> MGFSAEQAKKDGKDQSPVSESSSVGGTSPATASSVVSPNEPKLSGKEAKALKKARKQASRRAKAEAAAANNPPGVSEEKKVAIPNKNSNQQKKASKQNPQNSPETDANLQEKKIFEEKQVSIFSHLDWRRRRTTENIPKDIHPAVIRLGLKLANYKIFGSNQRCIDLLKTFKIVIQDYQTPYGTTLSRHLTTHINSQIAYLVSTRPLSISMGNAIRFLKLEISVLDIDLTDDEGKELLLEKIDSYIRDRIIIAGQVIVQAATEKIQDGDVILTYLHSSTVNDVLIHAKNVGKKFRVVVVDSRPEFEGRVCLKLLTEHGIECTYVMISALSYIMQEVTKIFLGGHAMLSNGALYSRAGTSLISLLGHESNVPVIACCESYKFTERIQLDSLVYNELAPGDQLVNMGVDDFEEKPGVLANWKSVKNLKLLS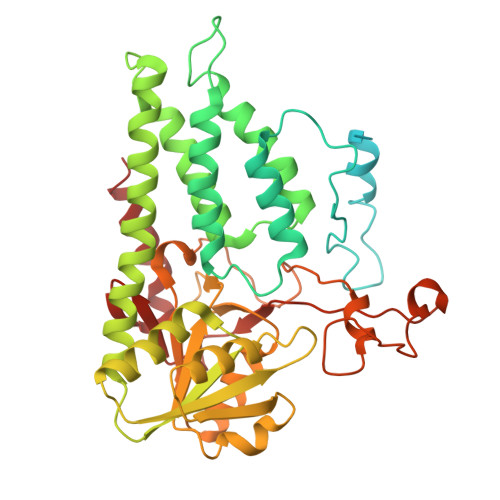LKYDVTPPRLITVCVCEMGLLPSTSVPAIINEFKQVYA> MGGEVEKIVREAARAAREG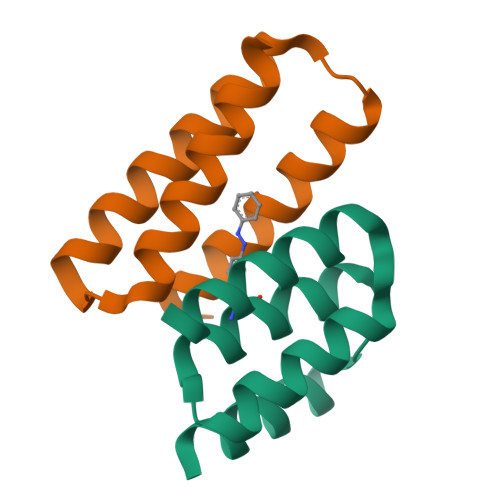DKEKLKELLAEAVAKGYVEATKFIAELALKAGAITKEEKAKYIAKAENGSHHHHHH;> MGAVERLAEKAYELLKLVKEAAPLEEVKELADEIIAEAEAALAEKPSVELKVILELAKELLEEAEK> KWPEPVFGRLVSPGFPEKYGNHQDRSWTLTAPPGFRLRLYFTHFNLELSYRCEYDFVKLTSGTKVLATLCGQESTDTERAPGNDTFYSLGPSLKVTFHSDY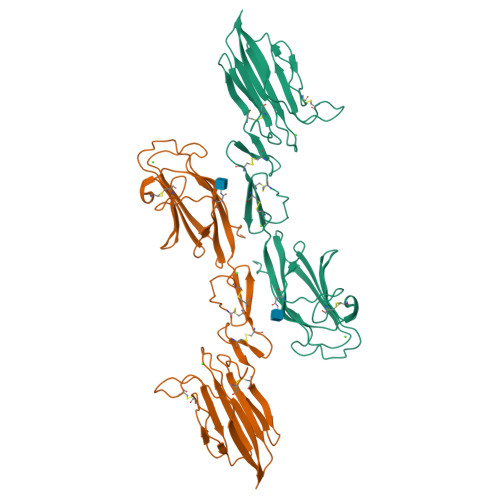SNEKPFTGFEAFYAAEDVDECRTSLGDSVPCDHYCHNYLGGYYCSCRVGYILHQNKHTCSALCSGQVFTGRSGFLSSPEYPQPYPKLSSCAYNIRLEEGFSITLDFVESFDVEMHPEAQCPYDSLKIQTDKREYGPFCGKTLPPRIETDSNKVTITFTTDESGNHTGWKIHYTSTAQ>[24x]MSTFPIDSGARIGEMKRVTKETNVSVKINLDGTGVADNSSGIPFLDHMLDQLASHGLFDVHVKATGDTHIDDHHTNEDVALAIGTALLQALGDRKGINRFGNFSAPLDEALVHVSLDLSGRPHLGYDLNIPTQRVGKYDTQLVEHFFQSLVNTSGMTLHIRQFSGTNSHHIIEATFKAFARALRQATEYDTRRRGTIPSSKGVLSRS

Plant HISN5 catalyzes the sixth step of the HBP, in which imidazole-glycerol phosphate (IGP) is dehydrated to form imidazole-acetol phosphate (IAP). The MtHISN5 subunit contains a four α-helix bundle sandwiched between two β-sheets whose four strands are almost perpendicular to each other. In solution, MtHISN5 forms a homo 24-mer with octahedral (432) symmetry of approx. 110 Å diameter and a total mass of 540 kDa. The dimensions of the MtHISN5 oligomer did not change significantly after the binding of IG2, indicating a lack of major conformational rearrangements. The active site of MtHISN5 (see below) contains two Mn2+ cations (Mn1 and Mn2) bound by residues belonging to different subunits.

The crystal structures cover the MtHISN5 sequence starting from Gly77 or Ala78 through Arg260/261 (chain and structure-dependent). Both cryoEM structures (unliganded and IG2 complex) have been reconstructed from EM maps with octahedral symmetry, and therefore contain 24 identical protein chains, spanning from Ala78 to Arg261 (IG2 complex) and Arg262 (unliganded). The cryoEM and crystal structures share the same pattern of Mn2+ coordination. The Mn2 coordination sphere is incomplete in the MtHISN5-unliganded cryoEM structure, owing to the lower map resolution. The corresponding position is occupied by a water molecule in the unliganded cryoEM structure or by the imidazole moiety in the MtHISN5-IG2 complex. To this end, we studied the cryoEM MtHISN5-unliganded structure in the Caver Analyst 2.0 and Caver 3.0.3 PyMol plugin (Chovancova et al., 2012; Jurcik et al., 2018). Most of the tunnels are distributed along the 2-, 3-, and 4-fold axes. The average diameter of the tunnels along the 2-fold axes is large enough to allow infiltration only by very small molecules (< 60 Da), such as EDO, FMT, and water. Larger molecules, however, could permeate the inner cavity of MtHISN5 through the tunnels along the 3-fold and 4-fold axes, which are approximately 2.5 times wider in diameter.> MSAKDERAREILRGFKLNWM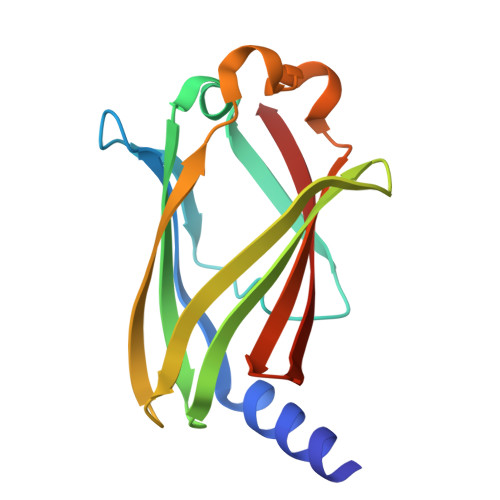NLRDAETGKILWQGTEDLSVPGVEHEARVPKKILKCKAVSRELNFSSTEQMEKFRLEQKVYFKGQCLEEWFFEFGFVIPNSTNTWQSLIEAAPESQMMPASVLTGNVIIETKFFDDDLLVSTSRVRLFYV> SNAMRIVAP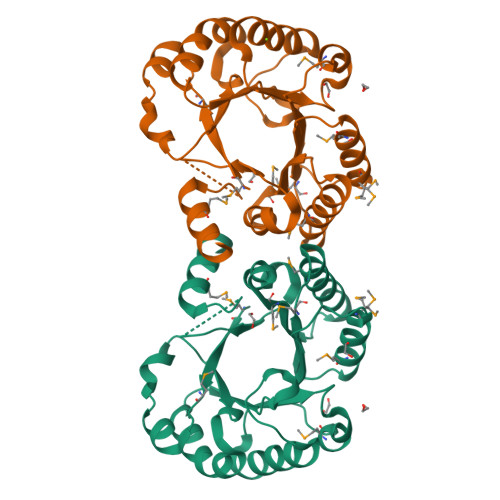VMPRHFDEAQAIDISKYEDVNLIEWRADFLPKDEIVAVAPAIFEKFAGKEIIFTLRTVQEGGNITLSSQEYVDIIKEINAIYNPDYIDFEYFTHKSVFQEMLDFPNLILSYHNFEETPENLMEAFSEMTKLAPRVVKIAVMPQSEQDVLDLMNYTRGFKTLNPEQEFATISMGKLGRLSRFAGDVIGSSWTYVSLDHVSGPGQVTLNDMKRIIEVLEMDISN> AGGGAAAAGGGGAGGGAAA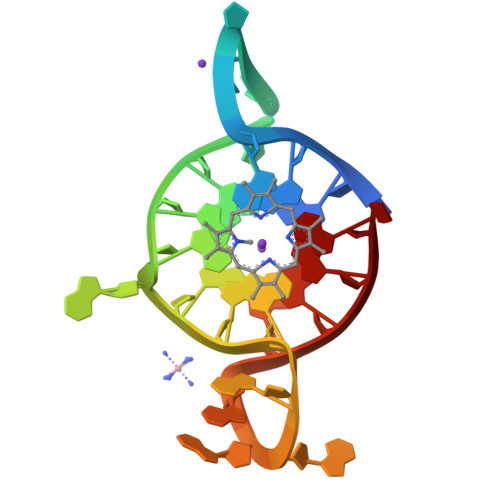AGGGGA> MFQKQVYRQYTPGFPGDLIEDGPKRARPGRIMSLSAVNPAATATGPNRASRAFGYAG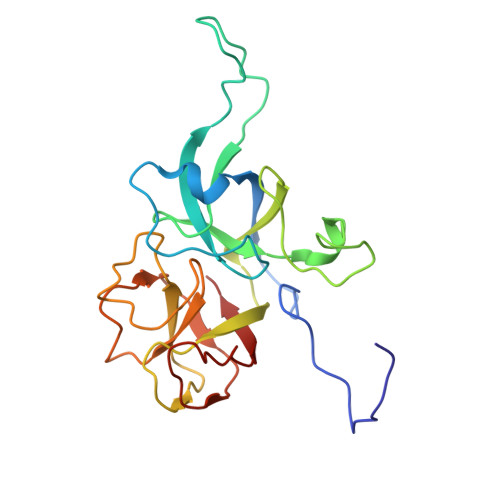DVSALGEGQPKTIAARASEVVIGGANFFGVLGHPKHYALFGSAGDSLAPSYDLPDGAEGEFFDMATGLVVEIFNGAAAALDLDYGDLVAYVPNNLATADDALGLPAGALVGFKTGSMPTGLVQIPNARIVNAISLPAQSAGNLVAGVTIVQLTQ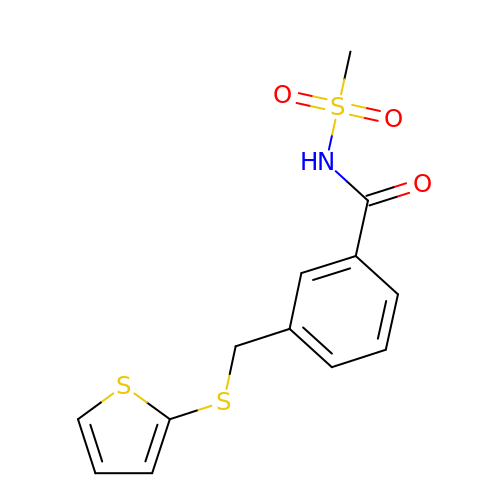N-(methylsulfonyl)-3-{[(thiophen-2-yl)sulfanyl]methyl}benzamide | C13 H13 N O3 S3 | VUNXNZBHBBHTIB-UHFFFAOYSA-N>MLRAKVRRIALANQKGGVGKTTTAINLAAYLARLGKRVLLVDLAPQGNATSGLGVRAERGVYHLLQGEPLEGLVHPVDGFHLLPATPDLVGATVELAGAPTALREALRDEGYDLVLLDAPPSLSPLTLNALAAAEGVVVPVQAEYYALEGVAGLLATLEEVRAGLNP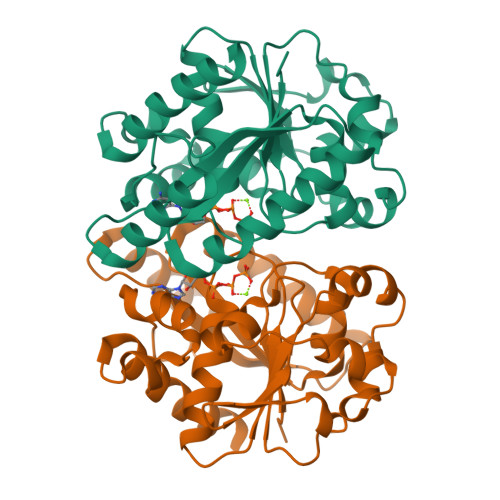RLRLLGILVTMYDGRTLLAQQVEAQLRAHFGEKVFWTVIPRNVRLAEAPSFGKTIAQHAPTSPGAHAYRRLAEEVMARVQEAGSHHHHHH[4x]>[2x]MAVRTKTLDKAGVLHRTKTADKGKRLRKKHWSASW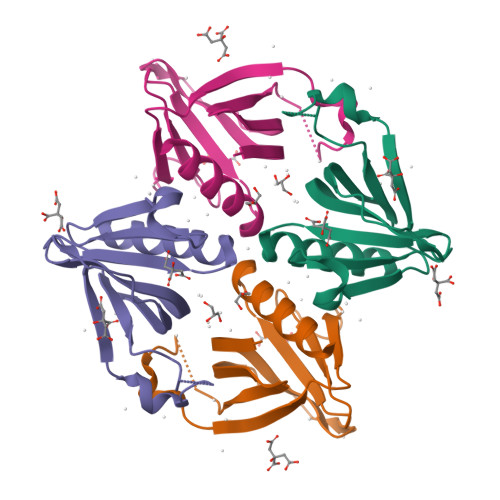TVLEGGVLTFFKDSKTSAAGGLRQPSKFSTPEYTVELRGATLSWAPKDKSSRKNVLELRSRDGSEYLIQHDSEAIISTWHKAIAQGIQE>MVNEVIDINEAVRAYIAQIEGLRA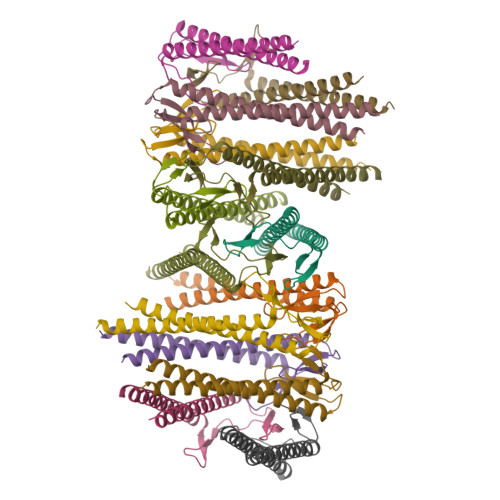EIGRLDATIATLRQSLATLKSLKTLGEGKTVLVPVGSIAQVEMKVEKMDKVVVSVGQNISAELEYEEALKYIEDEIKKLLTFRLVLEQAIAELYAKIEDLIAEAQQTSEEEKAEEEENEEKAE[14x]> MIAPLILYLDVPFTTFRESHAREMGKTYPVPPPATVYGMLLSLVGETNVYRHCGVELAIAMLSSPKKSRILRQMRRFKNADFSHPENVIPCYQEILSNLKCLIWVRSDEEKIQPSLRERIQLAFDHPELVRRFGCLFLGESDQLIKTIKLAREDYLEGVRQWAIRDNRGRLTLPYWVDHVGSRNTRFLRYRIEEMDRLSPPDLAWTMVQSPI;> MTAILIQSEEYVDLTFKLRGAPIPLDNGYLTYAALSRICPPLHELKSIGIHPIAGIPTRNNLLELTAQSRLKIRIYHQQIPLIYPYLAGQAFHIGQNFYQLDIPDYKPLISSESVYSRLVIIKGFQDSTNFIEAVQRQMDNLGIQGKIELLTRQDGTPQRRQLTINKEGKQFKVRGFGVKISELNPEDSLTLQEQGIGGKRKMMCGIFVPATRSKEEEET;>MMTQKKNDSNIPNYYLYGTVLTRYGLASLNHDIRRGNKTILQKGYWNNGKIHSFVGSSAIRWALRFYLQKQGYLVNRVWDEEEHINRLTSEDFDPEKFYDDDIFGFALLESAETEEDTSTTKRKKKQTKTSTPNQRMGALGMNMAVSLTPYDGAVKLGAKSGREKDSTSLHFTEYHATRYQYYFGIDATHLKDFSRILPMIDGIMNLPKVGGSSNIFNYPFCPDSLVFQWTNHFASYISYCFEYCDPKSKEAKLSQEFIDEVECGQIDPSKLWIGGTIVKDLQQLDNFESSPLNKAHIYRNRNEMIEALKTVIKRDLGLEESK[6x];> MHHHHHHHHIVSTQPKISLSLHAADTTIMHRVGMTGLYMTLKRLEKQYPLSRQRGGHISWFLTADTIELFWEGSDFIALSWLINESFQLDDTGLIHLVGLDNDRIDLRQKIHIHEGICGVFLRLNKFYQAGEIINTELRFEEKQVEYQYKSLTWYAHQTFAEKLCEADTQQLRHDYIQITSWLYLGGIVRHARTQNTTKLEEKPEYALALLFVPVVCHYCLLHIPSEDLKERKPHRYLVVIPEIKDFEDASQRRWRLQQLETKQFHVSSLGEAGLLYYSLDDIQPEVAYYQACQVWLYEKTNKASRQRTLMSIEEIKIDKNILITYQQVQKYFKTNYQIIKYKQIFIKVNPIRSLIADNLVKGIHWWSNFWEKLVIEDSKEYLFNQLFSNREGFIIMAENSEEDKQYLIFIKVFQQAMKGNFAKIYAKTEEGKDPPI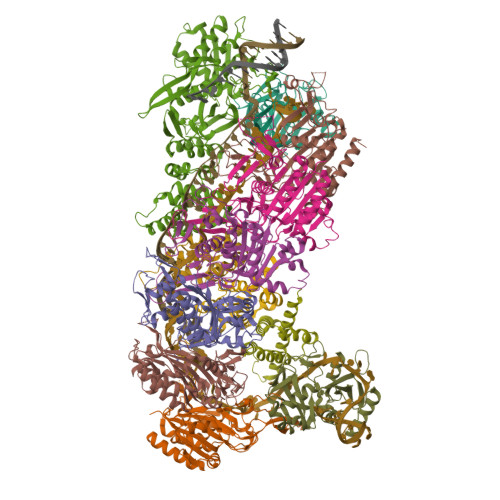KKKVERLRAELNYCYDELSFKEYLSDFLVRGGLNKYFNEHQEEIALLIKKSPWQEIRIWSLLAIASYKPKDKLTNRDDSSLSNNQKLEEVNDDSEEE;>MAENSEEDKQYLIFIKVFQQAMKGNFAKIYAKTEEGKDPPIKKKVERLRAELNYCYDELSFKEYLSDFLVRGGLNKYFNEHQEEIALLIKKSPWQEIRIWSLLAIASYKPKDKLTNRDDSSLSNNQKLEEVNDDSEEE[3x]>MAHHHHHHSGTVTDDYLANNVDYASGFKGPLPMPPSKHIAIVACMDARLDVYRMLGIKEGEAHVIRNAGCVVTDDVIRSL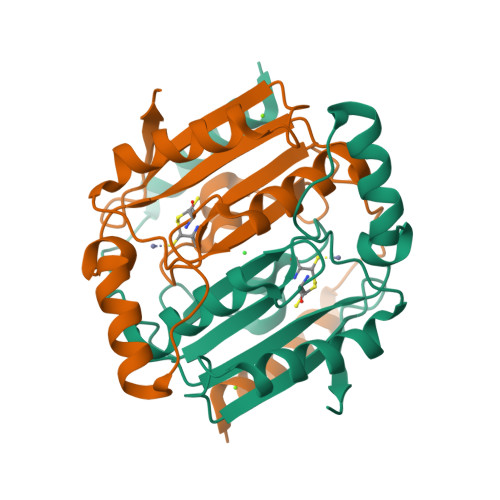AISQRLLGTREIILLHHTDCGMLTFTDDDFKRAIQDETGIRPTWSPESYPDAVEDVRQSLRRIEVNPFVTKHTSLRGFVFDVATGKLNEVTP[4x]>[2x]MSSDAISLRAAGPGDLPGLLELYQVLNPSDPELTTQEAGAVFAAMLAQPGLTIFVATENGKPVATATLLIVPNLTRAARPYAFIENVVTLEARRGRGYGRTVVRHAIE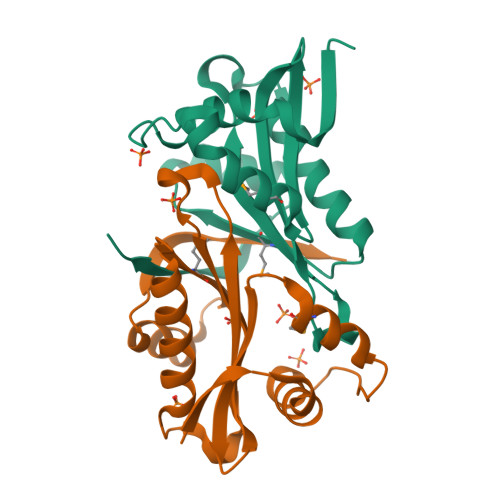TAFGANCYKVMLLTGRHDPAVHAFYESCGFVQNKTGFQIRQD>EAPFTLKVNTLPLNFDKAEHHRKFQI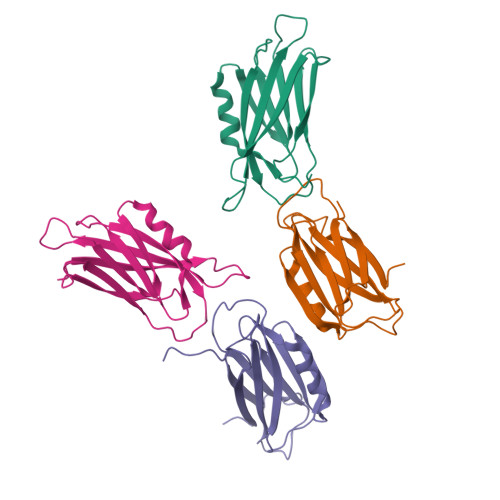HINVSYIGERPNSNMVIVDVKMVSGFIPVKPSVKKLQDQSNIQRTEVNTNHVLIYIEKLTNQTMGFSFAVEQDIPVKNLKPAPVKVYDYYETDEFAIEEYSAPFSSDS[2x]> MLDNFNQPKGSTIGVLKDGRTIQEAFDSLPRLESFSGSTATDKLRAAITLGVSEVAIGPVEGNGGRPYEFGDVVIPYPLRIVGCGSQGINVTKGTVLKRSAGASFMFHFTGEGQAQRPMGGGLFNINLNGDTATALGDIIKVTQWSYFK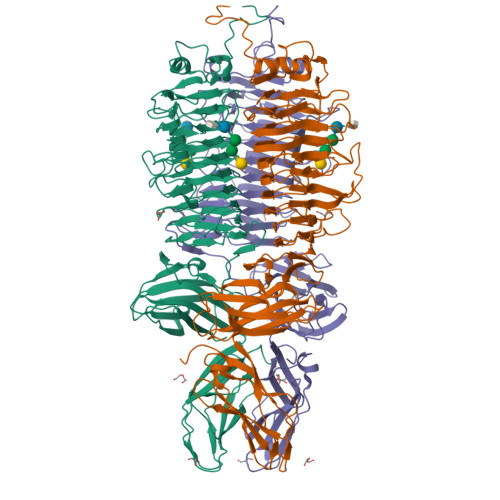ANNCAFQNMAGWGIRLKDVMESNISGNLFRRLGGPSGGGILFDDVRSAVTDNVNNLHIEDNTFALMSGPWIGSTANSNPDLIWIVRNKFEFDGTPAAPNTVDSYVLDFQQLSRAFIQDNGFTHFTTERNRYVGVLRVGATAVGTIKFEDNLLFACESAGLIAGGIVVSRGNVNNQGSATTAIKQFTNTSSKLCKLERVINVQSNGNVSVGQQILPDGYINMAELPGNTRLPSEYDADGETTSVLRVPANTQVRQWSVPKMYKDGLTVTKVTVRAKGAAAGAILSLQSGSTVLSTKSIDAGVWKNYVFYVKANQLQETLQLRNTGTADVLADGMVFGKVDYIDWDFAIAPGTLAAGAKYTTPNQSYLDVAGMRVQAVSIPMFDGPTTGLQVWVEATSANGSFVVVMKNDTGSELVTTVTRCRVRAFVSKGHHHHHH>MAASITAITVENLEYPAVVTSPVTGKSYFLGGAGERGLTIEGNFIKFTAIGVYLEDIAVASLAAKWKGKSSEELLETLDFYRDIISGPFEKLIRGSKIRELSGPEYSRKVMENCVAHLKSVGTYGDAEAEAMQKF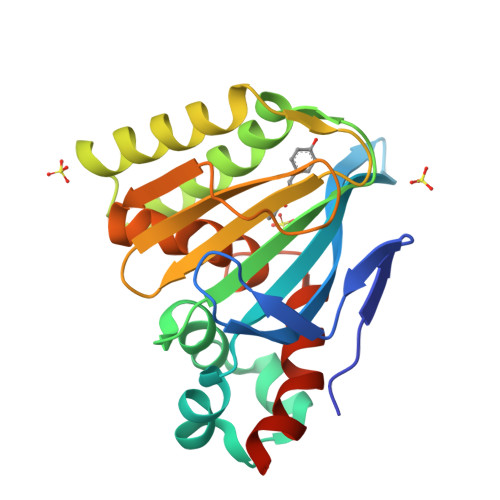AEAFKPVNFPPGASVFYRQSPDGILGLSFSPDTSIPEKEAALIENKAVSSAVLETMIGEHAVSPDLKRCLAARLPALLNEGAFKIGN[2x]(2S)-2-(acetylamino)-N-methyl-4-[(S)-methylsulfinyl]butanamide 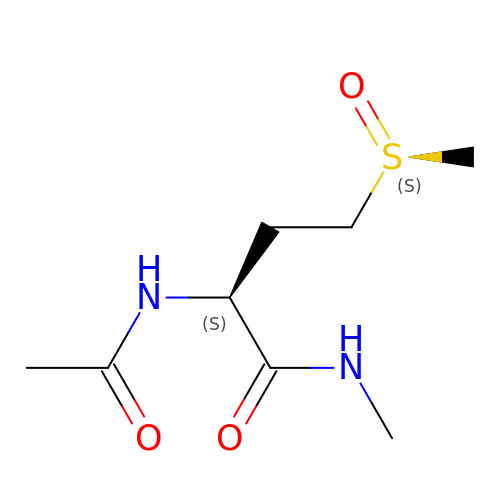| C8 H16 N2 O3 S | HOKSMYPIXLKSMM-WJWGPLDTSA-N> MVSLLRRTFSEEIKEELVNVPFGSREEVISELLGFIKARGDLDVKSRHIVFSLHSFAASRRLLNLMKYLSKPVSEIIVEKSHNIKKRYIKITAEYSESFMVIEPFFDVALFVSFLRGLFLSGGSMTNPRYHYHLEINLFEEETLALTRKSLKDFFNINAGIIELRNTRKLYIKSIKDILVFLEAIGVQRKLEEIDRIVTERKVIGDVNRTVNFIEANAIRTANSTARQIRAIELIKENMGLENLPEDLRRVALVRLRNKELSLRELGKKLNLT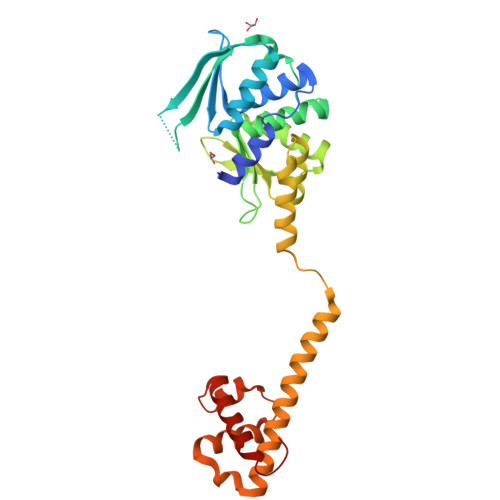KSQIYSKLKRIIKIAERFGDVK>[2x]ILVRKNIHSLSHHEAEELRDALYKLQNDESHGGYEHIAGFHGYPNLCPEKGDEKYPCCVHGMSIFPHWHRLHTIQFERALKKHGSHLGIPYWDWTQTISSLPTFFADSGNNNPFFKYHIRSINQDTVRDVNEAIFQQTKFGEFSSIFYLALQALEEDNYCDFEVQYEILHNEVHALIGGAEKYSMSTLEYSAFDPYFMIHHASLDKIWIIWQELQKRRVKPAHAGSCAGDIMHVPLHPFN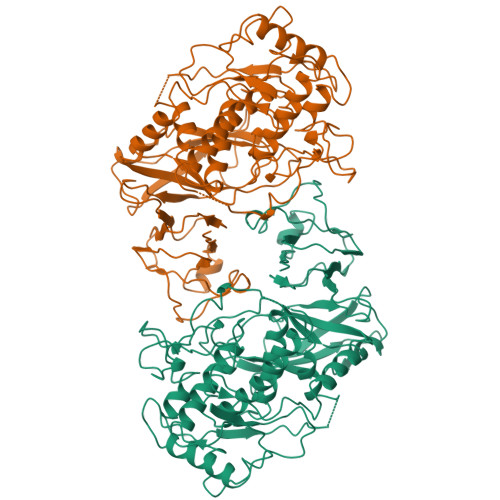YESVNNDDFTRENSLPNAVVDSHRFNYKYDNLNLHGHNIEELEEVLRSLRLKSRVFAGFVLSGIRTTAVVKVYIKSGTDSDDEYAGSFVILGGAKEMPWAYERLYRFDITETVHNLNLTDDHVKFRFDLKKYDHTELDASVLPAPIIVRRPNNAVFDIIEIPIGKDVNLPPKVVVKRGTKIMFMSVDEAVTTPMLNLGSYTAMFKCKVPPFSFHAFELGKMYSVESGDYFMTASTTELCNDNNLRIHVHVD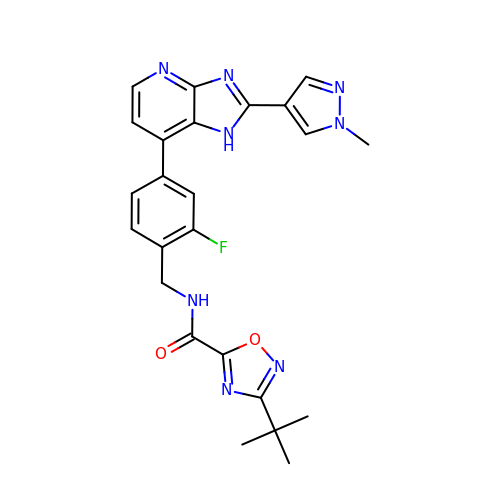3-tert-butyl-N-({2-fluoro-4-[2-(1-methyl-1H-pyrazol-4-yl)-1H-imidazo[4,5-b]pyridin-7-yl]phenyl}methyl)-1,2,4-oxadiazole-5-carboxamide | C24 H23 F N8 O2 | KHIWVHWOVLFXIZ-UHFFFAOYSA-N>[2x]MNNQG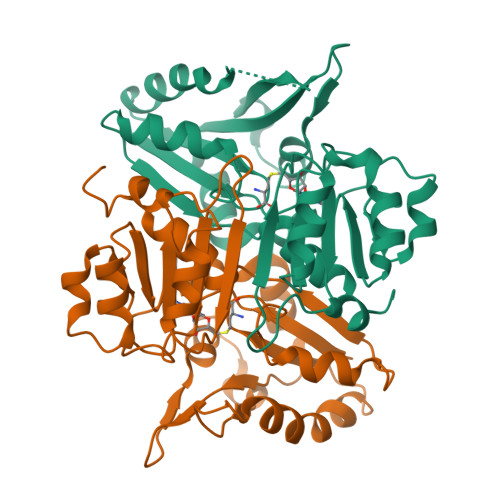SIISVSLGPGDPGLITVKALSQLREADVIYYPGTVSASGAVTSVALDILKEFDLDPSKLRGMLVPMSRSRGAAEASYAANYASMAEEVQAGRRVAVVSVGDGGFYSTASAIIERARRDGLDCSMTPGIPAFIAAGSAAGMPLALQSDSVLVLAQIDEIGELERALVTHSTVVVMKLSTVRDELVSFLERYAKPFLYAEKVGMAGEFITMEVDALRSRAIPYFSLLVCSPHCRQSTLSPFASKLAAALEHHHHHH>SQEFRSYTGEGNNKQNPKQGSIFTPFIRLANPIKFNKNGFPNITNQPSRAISNIIFDQQTHIGSKEHLTDMFNMWGQFLIHNMALSKPEPNSWPIKVPKCDQYFDPACIGNKTMNYFRTRATEVPCDVGKTVVDEDGKCYEQINSLGSYIDGNVLYGNSEEICKNLRSLSGGEMKMTVTDVGDLPPKNVPGVPMDNDANLFPIDQLYSVGERRGNENPGLLSIHTLLLRDHNRLARKFARLHPEWDDERVFQQSRSCIIEQIQKITYDEYLPTTLGSFPSYTGYDANVNAQVSNEFTTTAFRFGHSEVGPFMEYYSENGTRLQPLPIKFSYFNPHALNRGVEPLIRGLIINEEENIDIYMISDLRNFLFGKPGQGGLDLASRNLQRNR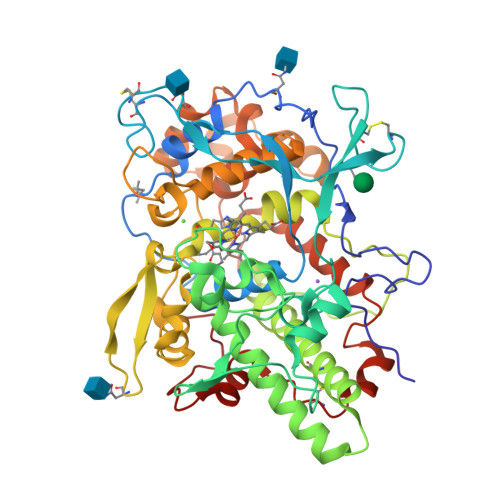DHGIPPYNSLRRQLGLRPVQTWSDITSDPQIQNRLKNAYKSVDDIDSYVGGLAEDHMEGSCVGQTFYLIIYEQFFRTRAGDRFWYETPEMRMVNRECETTTFAEVIKRTTSNIGYVQPNVFRK[2x]>GMDPNEAVREFAKEIDVSYVKIEEVIGAGEFGEVCRGRLKAPGKKESCVAIKTLKGGYTERQRREFLSEASIMGQFEHPNIIRLEGVVTNSMPVMILTEFMENGALDSFLRLNDGQFTVIQLVGMLRGIASGMRYLAEMSYVHRDLAARNILVNSNLVCKVSDFGLSRFLEENSSDPTETSSLGGKIPIRWTAPEAIAFRKFTSASDVWSYGIVMWEVMSFGERPYWDMSNQDVINAIEQDYRLPPPPDCPTSLHQLMLDCWQKDRNARPRFPQIVS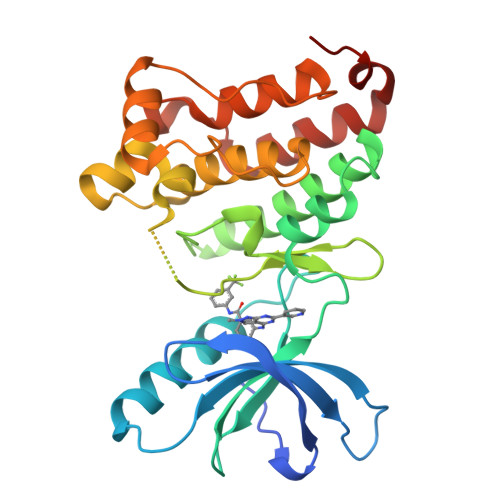ALDKMIRNPASLKIVARENG[2x]>MGIVPTLQNIVATVTLGCRLDLKTVALHARNAEYNPKRFAAVIMRIREPKTTALIFASGKMVVTGAKSEDDSKLASRKYARIIQKIGFAAKFTDFKIQNIVGSCDVKFPIRLEGLAFSHGTFSSYEPELFPGLIYRMVKPKIVLLIFVSGKIVLTGAKQREEIYQ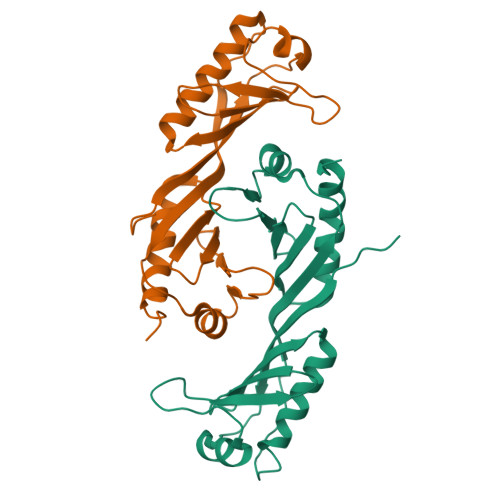AFEAIYPVLSEFRKM[2x]>[4x]TTKDEIEK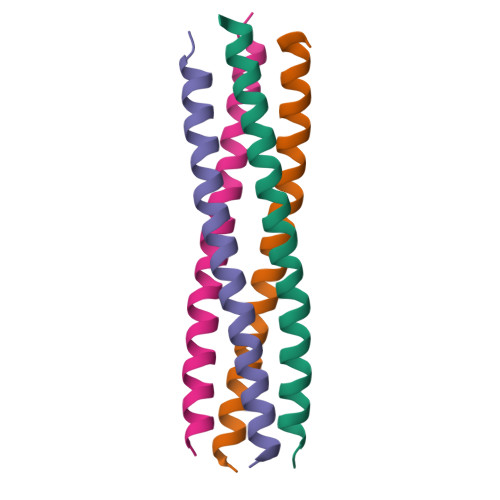QMDRVVKEMRRQLEMIDKLTTREIEQVELLKRIHDKLVVQSTG A widely applicable approach is the use of photocaged substrates, where the photocage is soaked into the crystal in advance and then activated using a laser pulse to provide uniform initiation of the reaction throughout the crystal. This work characterizes photocage release of nitric oxide and binding of this ligand to two heme protein systems, cytochrome c′-β and dye-decolourizing peroxidase B using a fixed target sample delivery system. In this work, we describe a thorough characterization of the application of the NO photocage N,N′-bis-(carb­oxy­methyl)-N,N′-di­nitroso-1,4-phenyl­enedi­amine (henceforth referred to as NO cage) to room-temperature microcrystals of two proteins: a gas binding cytochrome c′ (McCP-β) and a dye-decolourizing peroxidase B (DtpB). Laser parameters for photoactivation are systematically explored, and time-resolved structures over timescales ranging from 100 µs to 1.4 s using synchrotron and XFEL beamlines are described. We have demonstrated a sample and time efficient approach using fixed targets to carry out time-resolved SSX and SFX experiments with an NO photocage over the microsecond to second time regimes.

Comparison of these different structures revealed no significant changes in the binding geometry of NO or nearby residues in the heme pocket, meaning that only a two-state transition between unbound and bound states is observed. This suggests that any intermediate steps in the NO binding process must be complete on timescales of less than 100 µs. On binding to the heme, NO was observed to bind in an end-on fashion via the nitro­gen atom with an Fe—N distance of approximately 2.0–2.5 Å and an Fe—N—O angle of approximately 105–150°. The variability in these values occurs across the six independent heme groups within the crystallographic model and could represent either genuine differences in binding due to subtle differences in the crystalline environments or simply uncertainty in modelling a small ligand into the electron density features. A small shift in the side-chain position of Asn245 was observed compared with the ‘empty’ site structure in all six of the hemes, and at all laser powers and timepoints. For DtpB, the structure of the NO ferric heme complex of this or any other B-type DyP have not been previously determined, and thus we have demonstrated here that such a complex rapidly forms on exposure to NO after photocage release.

>[6x]EPEPQMVLSPLTSAAIFLVVTIDSGGEDTVRDLLSDVASLERAVGFRAQPDGRLSCVTGIGSEAWDRLFSGARPAGLHPFRELDGPVHRAVATPGDLLFHIRASRLDLCFALATEIMGRLRGAVTPQDEVHGFKYFDERDMLGFVDGTENPTGAAARRAVLVGAEDPAFAGGSYAVVQKYLHDIDAWEGLSVEAQERVIGRRKMTDVELSDDVKPADSHVALTSVTGPDGSDLEILRDNMPFGSVGREEFGTYFIGYARTPEVTETMLERMFLGTASAPHDRILDFSTAVTGSLFFTPAADFLEDLS> MAKQYDSVECPFCDEVSKYEKLAKIGQGTFGEVFKARHRKTGQKVALKKVLMENEKEGFPITALREIKILQLLKHENVVNLIEICRTKASPYNRCKGSIYLVFDFCEHDLAGLLSNVLVKFTLSEIKRVMQMLLNGLYYIHRNKILHRDMKAANVLIT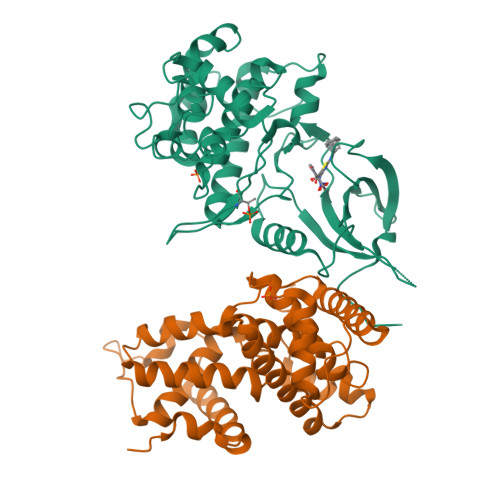RDGVLKLADFGLARAFSLAKNSQPNRYTNRVVTLWYRPPELLLGERDYGPPIDLWGAGCIMAEMWTRSPIMQGNTEQHQLALISQLCGSITPEVWPNVDNYELYEKLELVKGQKRKVKDRLKAYVRDPYALDLIDKLLVLDPAQRIDSDDALNHDFFWSDPMPSDLKGMLST;> MEGERKNNNKRWYFTREQLENSPSRRFGVDPDKELSYRQQAANLLQDMGQRLNVSQLTINTAIVYMHRFYMIQSFTRFPGNSVAPAALFLAAKVEGQPKKLEHVIKVAHTCLHPQESLPDTRSEAYLQQVQDLVILESIILQTLGFELTIDHPHTHVVKCTQLVRASKDLAQTSYFMATNSLHLTTFSLQYTPPVVACVCIHLACKWSNWEIPVSTDGKHWWEYVDATVTLELLDELTHELLQILEKTPNRLKRIWNWR> MIVFVRFNSSYGFPVEVDSDTSILQLKEVVAKQQGVPADQLRVIFAGKELPNHLT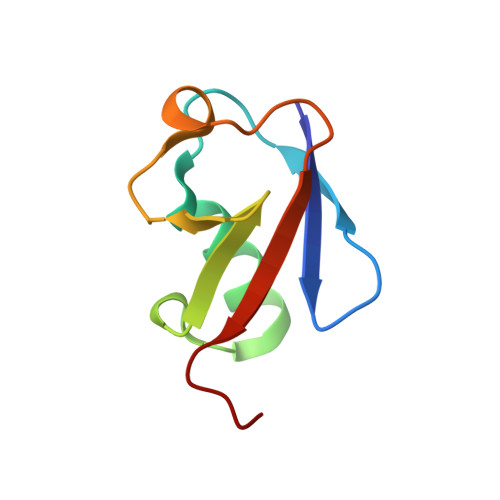VQNCDLEQQSIVHIVQRPRRR> QYDDDWQYEDCKLARGGPPATIVAIDEESRNGTILVDNMLIKGTAGGPDPTIELSLKDNVDYWVLLDPVKQMLFLNSTGRVLDRDPPMNIHSIVVQVQCVNKKVGTVIYHEVRIVVRDRNDNSPTFKHESYYATVNELTPVGTTIFTGFSGDNGATDIDDGPNGQIEYVIQYNPEDPTSNDTFEIPLMLTGNVVLRKRLNYEDKTRYYVIIQANDRAQNLNERRTTTTTLTVDVLDGDDLGPMFLPCVLVPNTRDCRPLTYQAAIPELRTPEELNPILVTPPIQAIDQDRNIQPPSDRPGILYSILVGTPEDYPRFFHMHPRTAELTLLEPVNRD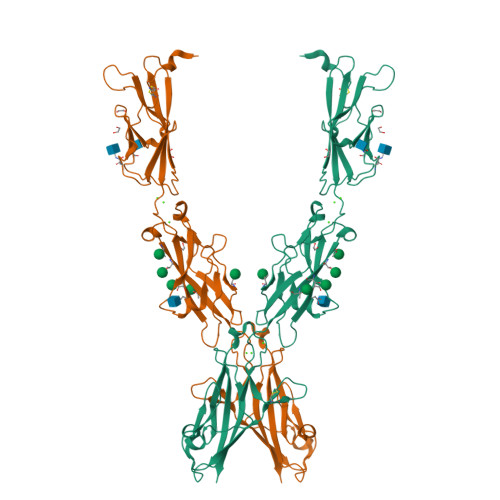FHQKFDLVIKAEQDNGHPLPAFASLHIEILDENNHHHHHHHH>MNNFGNEEFDCHFLDEGFTAKDILDQKINEVSSSDDKDAFYVADLGDILKKHLRWLKALPRVTPFYAVKCNDSKAIVKTLAATRTGFDCASKTEIQLVQSLGVPPERIIYANPCKQVSQIKYAANNGVQMMTFDSEVELMKVARAHPKAKLVLRIATDDSKAVCRLSVKFGATLRTSRLLLERAKELNIDVVGVSFHVGSGCTDPETFVQAISDARCVFDMGAEVGFSMYLLDIGGGFPGSEDVKLKFEEITGVINPALDKYFPSDSGVRIIAEPGRYYVASAFTLAVN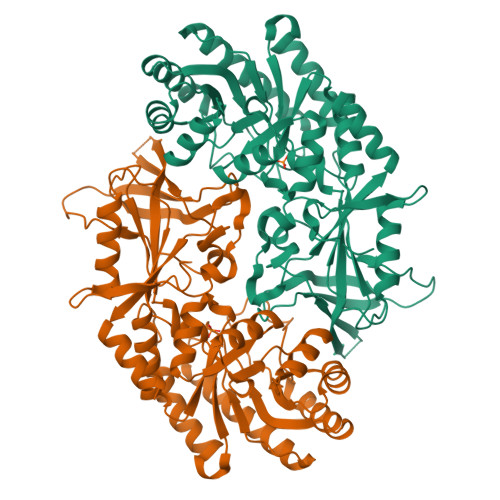IIAKKIVLKEQTGSDDEDESSEQTFMYYVNDGVYGSFNCILYDHAHVKPLLQKRPKPDEKYYSSSIWGPTCDGLDRIVERCDLPEMHVGDWMLFENMGAYTVAAASTFNGFQRPTIYYVMSGPAWQLMQQFQNPD[2x]>[2x]SMKRGRGGRVDPFEFVTYSGEEIKESSSEERVKEGANKSSPTRTRILSAALSPAERAIFDVPIEKWLSIDRSSLSGWKCAVPRPVTIEQLRPVDPSDAILRHIALYRGPVTDLQLDAIVNAANTRCLGGGGVDGAIHRVAGPLLLRECATFNGCQTGECRLTKGYQLPARYVLHTVGPVGERPDMLRKCYRSILSLALKNGLRSIGFCCVSTGVYGYPLLPATRIALGETRKFLEEHGGALDMCCFACFQEDEYKTYEKCVGKSSL

We named these proteins as Trypanosoma brucei MacroD-like protein (TbMDO) and Trypanosoma cruzi MacroD-like protein (TcMDO). We show that the trypanosomatid MacroD1/MacroD2 homologues are hydrolyzing both protein-linked ADP-ribose and free O-acetyl-ADP-ribose. The macrodomain fold (starting from residues 99 and 92 in TbMDO and TcMDO, respectively) is well-conserved between the human MacroD proteins and consists of a central mostly parallel six-stranded β-sheet surrounded by five α-helices. Active site of the macrodomains is located at the C-terminal edge of the β-sheet and is lined by N-terminal ends of four α-helices.

Crystal structures of TbMDO were determined to 1.95 Å and 1.2 Å resolution (for crystal form 1 and 2, respectively) and crystal structure of TcMDO to 2.0 Å resolution. The two crystal forms of TbMDO are almost identical with RMSD of 0.4 Å. Structures of TbMDO and TcMDO comprise residues from 11–261 and 13–257, respectively and share a highly conserved structure (RMSD 0.84 Å). While the N-terminus of the TbMDO folds back to the core and extends the β-sheet, the N-terminus of the TcMDO packs to the precisely same site but in the neighboring molecule in the crystal. When comparing the ADP-ribose bound structure to apo-TbMDO, it is evident that the binding site for ADP-ribose in TbMDO is preformed. Upon binding of ADP-ribose, eight water molecules (and a glycerol molecule) are displaced but no large conformational changes in coordinating residues are observed.>[3x]GSSGSSGMQIGKIIKVSGPLVMAENMSEACIQDMCLVGDLGVIGEIIEMRQDVASIQVYEETSGIGPGEPVRSTGEALSVELGPGIISQMFDGIQRPLDTFMEVTQSNFLGRGVQLPALDHEKQWWFEATIEEGTEVSAGDIIGYVDETKIIQHKIMVPNGIKGTVQKIESGSFTIDDPICVIETEQGLKELTMMQKWPVRRGRPIKQKLNPDVPMITGQRVIDTFFPVTKGGAAAVPGPFGAGKTVVQHQIAKWSDVDLVVYVGCGERGNEMTDVVNEFPELIDPNTGESLMERTVLIANTSNMPVAAREASIYTGITIAEYFRDMGYDVAIMADSTSRWAEALREMSGRLEEMPGDEGYPAYLGSRLAEYYERSGRVIALGSDQREGSITAISAVSPSGGDISEPVTQNTLRVVKVFWGLDSSLAQKRHFPSINWIQSYSLYSTEVGRYMDQILQQDWSDMVTEGMRILQEEEQLNEIVRLVGIDSLSDNDRLTLEVAKSIREDYLQQNAFDDVDTFTSREKQFNMLKVILTFGKEARKALSLGAYFNEIMEGTVAVRERISRSKYIPEEELAKISSINEEIKETIQLIVSEGGMTDD;>[3x]GSSGSSGMIKEYRTIKEVVGPLMAVEKVSGVKYEELIEVRMQNGEIRRGQVLEVQEDKAMVQIFEGTSGICLKNSSVRFLGHPLQLGVSEDMIGRVFDGLGRPKDNGPEILPEKYLDINGEVINPIARDYPDEFIQTGISAIDHLNTLVRGQKLPVFSGSGLPHKELAAQIARQATVLDSSDDFAVVFAAIGITFEEAEFFMEDFRQTGAIDRSVMFMNLANDPAIERIATPRMALTAAEYLAYEKGMHVLVIMTDMTNYAEALREISAARREVPGRRGYPGYLYTNLATLFERAGRIRGLKGSVTQIPILTMPEDDKTHPIPDLTGYITEGQIILTRELYKSGIQPPIDVLPSLSRLKDKGTGAGKTREDHAATMNQLFAAYAQGKQAKELAVVLGESALSDID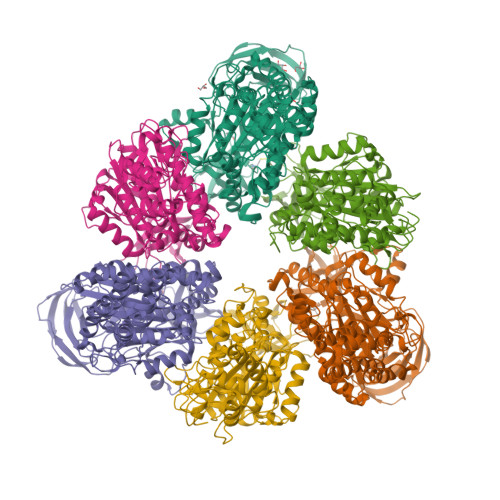KIYAKFAERFENEYVNQGFYTNRTITETLDLGWELLAMLPRTELKRIKDDLLDKYLPEGK> MSPILAHDVVKPQGVPVWAFQ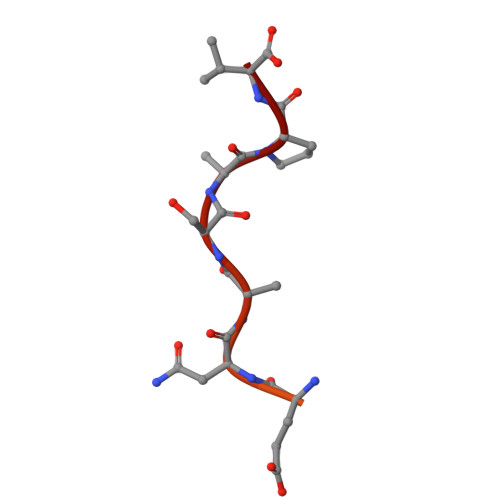AKDVENASAPV>[2x]MEQETLEQVHLTEDGGVVKTILRKGEGGEENAPKKGNEVTVHYVGKLESSGKVFDSSRER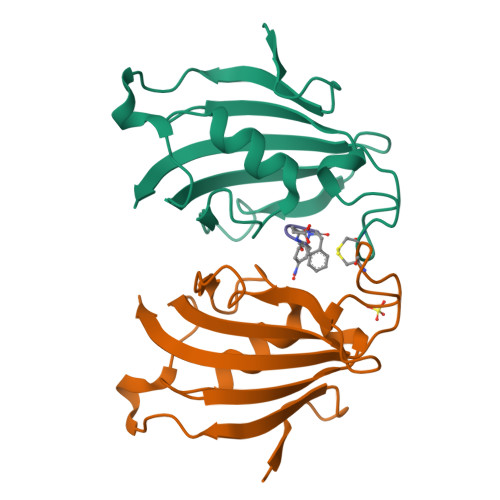NVPFKFHLGQGEVIKGWDICVASMTKNEKCSVRLDSKYGYGEEGCGESIPGNSVLIFEIELISFRE> DA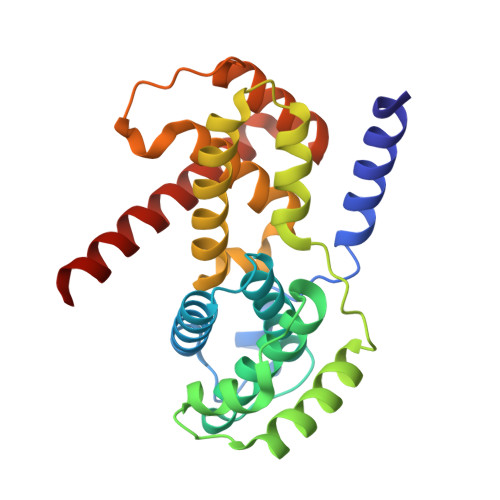NLLNDRVLRAMLKAEETCAPSVSYFKCVQKEVLPSMRKIVATWMLEVCEEQKCEEEVFPLAMNYLDRFLSLEPVKKSRLQLLGATCMFVASKMKETIPLTAEKLCIYTDNSIRPEELLQMELLLVNKLKWNLAAMTPHDFIEHFLSKMPEAEENKQIIRKHAQTFVALCATDVKFISNPPSMVAAGSVVAAVQGLNLRSPNNFLSYYRLTRFLSRVIKCDPDCLRACQEQIEALLESSLRQAQQNMD> MTVTITADVRDVTGQPDNQQWVFSTVLRQQDGSILTQKQVRVNPVDGALSVELEPGFAIVVYGEYRWFIEVPETDAGLWGLIATSVAVPPDTSAELLADAVNGYLDANPPSADWDALSNVPSEFPPSAHDHVAADVTDLDSAIAAYLASNPPEAGSVAWDDIDDKPSTFTPSSHTHSIANVTGLQDALDEKLDEAAVDARVSLGTAALVDSAPSTLDTLNELAAALGDDPNFATTVASQIGAKADKATTITAGTGLTGGGDLSANRTLNVSFGTSSTTACVGNDSRLSNTRTPTDGSVTNAKVASGAGIALSKLATGYVAGSDNSGARTLTIWVGTEAQYTAIGTKDSNTIYLRT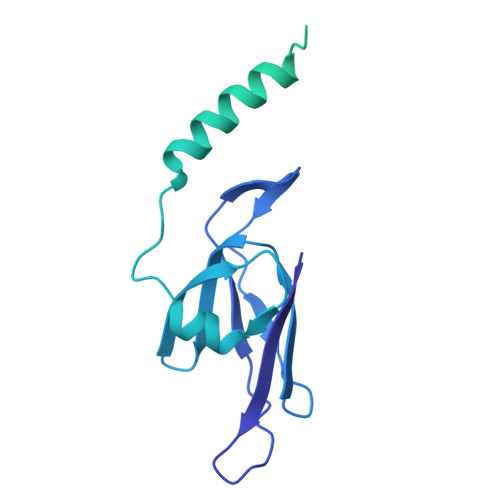A The ALDH enzymes catalyse the NAD(P)+-dependent irreversible oxidation of a wide spectrum of endogenous and exogenous aldehydes and are found in all subcellular regions including the cytosol, mitochondria, endoplasmic reticulum and nucleus, often being expressed in more than one compartment. In particular, three members of the cytosolic aldehyde dehydrogenase class 1 (ALDH1A1, ALDH1A2, ALDH1A3) have a key role in vertebrate development. Indeed, they show a high specificity for retinaldehyde that they oxidise to the potent differentiation factor retinoic acid (REA). Human ALDH1A3 has a key role in vertebrate development by participating in the synthesis of the differentiation factor retinoic acid40.

Here we report on the first crystal structure of the human ALDH1A3 complexed with REA and NAD+, which has been determined at 2.9 Å resolution. The final human ALDH1A3 model contains eight identical chains per asymmetric unit, arranged as two independent tetramers and a total of 63 solvent molecules. Each monomer binds one molecule of NAD+ and one molecule of the product REA. The crystal structure of ALDH1A3 reveals a tetrameric assembly with intimately associated monomers. The structure analysis confirms that ALDH1A3 shares high structural homology with all classes of ALDHs and folds into 13 α-helices, 19 β-strands and the connecting loops, arranged into three functional domains. An important feature revealed by our structural studies is the precise definition of the catalytic pocket that consists of a tunnel connecting the protein surface to the catalytic cysteine, and that likely also represents the pathway for substrate access and product release, as previously predicted for sheep liver and human ALDH1A1. In summary, we observed two different and linked conformations for the REA-NAD+ couple in two different monomers: the first showing the REA carboxylate pointing toward the C314 and the second showing the product conformation with the REA carboxylate moiety oriented toward the protein surface. REA binds to monomer D in a closed conformation, with its carboxyl group close to the active cysteine and extends its β-ionone and isoprenic chain moieties along the whole access-substrate tunnel. In monomer C, REA binds in an open conformation with its isoprenic and carboxylic moieties pointing to the opening of the catalytic tunnel toward the protein surface. A remarkable difference that we observe in the active site structure in monomers C and D regards the strictly conserved E280 that shows two different conformations.

>HHHHHHLESTSLYKKAGMATANGAVENGQPDRKPPALPRPIRNLEVKFTKIFINNEWHESKSGKKFATCNPSTREQICEVEEGDKPDVDKAVEAAQVAFQRGSPWRRLDALSRGRLLHQLADLVERDRATLAALETMDTGKPFLHAFFIDLEGCIRTLRYFAGWADKIQGKTIPTDDNVVCFTRHEPIGVCGAITPWNFPLLMLVWKLAPALCCGNTMVLKPAEQTPLTALYLGSLIKEAGFPPGVVNIVPGFGPTVGAAISSHPQINKIAFTGSTEVGKLVKEAASRSNLKRVTLELGGKNPCIVCADADLDLAVECAHQGVFFNQGQCCTAASRVFVEEQVYSEFVRRSVEYAKKRPVGDPFDVKTEQGPQIDQKQFDKILELIESGKKEGAKLECGGSAMEDKGLFIKPTVFSEVTDNMRIAKEEIFGPVQPILKFKSIEEVIKRANSTDYGLTAAVFTKNLDKALKLASALESGTVWINCYNALYAQAPFGGFKMSGNGRELGEYALAEYTEVKTVTIKLGDKNP[8x]~{N}-(4-aminophenyl)-2-azanyl-ethanamide | C8 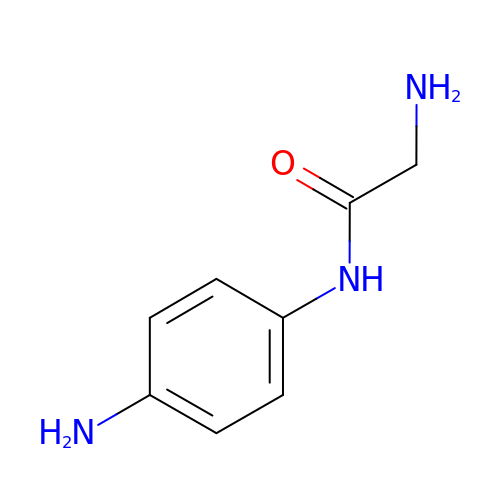H11 N3 O | DKCWGVIARWBMDV-UHFFFAOYSA-N Apicomplexan parasites, such as Plasmodium spp., rely on an unusual actomyosin motor, termed glideosome, for motility and host cell invasion. Actin filament capping proteins (CPs) are indispensable heterodimeric regulators of actin dynamics. CPs play a crucial role in actin dynamics by binding to the fast-growing barbed end of filamentous actin (F-actin) with high affinity in a Ca2+-independent manner, limiting protomer exchange to the pointed end. Despite retaining several characteristics of a canonical CP, the homodimeric Plasmodium berghei (Pb)CP exhibits crucial differences to the canonical heterodimers.

To gain structural insight into the unusual homodimerization of PbCPαα, we determined the structure of a C-terminally truncated PbCPαα homodimer (PbCPααΔC20), which was the only version of the parasite CPs that produced well-diffracting crystals, to 2.2-Å resolution. The two PbCPαΔC20 subunits form a structure that is less compact and intertwined than the canonical heterodimer, verifying earlier small-angle X-ray scattering (SAXS) and thermal stability analyses. Albeit being a homodimer, the structure is not completely symmetric. Thus, we will refer to chain A of the crystal structure as PbCPα1ΔC20 and chain B as PbCPα2ΔC20. Superposition of the two subunits reveals that structural deviations are mainly present at the dimer interface, possibly to accommodate complementary intersubunit interactions. In PbCPαΔC20, the presence of two identical stalk domains disrupts the formation of a compact structure. The 23-residue Plasmodium CPα-specific insert is located between the globule and cap β-sheets (Ser136–Ala159). The base of the insert is stabilized by a partial disulfide bond between Cys158 and Cys179 in the PbCPα1ΔC20 subunit but not in PbCPα2ΔC20. The H5 helix of PbCPα1ΔC20 is broken at His267 and turns back towards the same subunit in a β-hairpin-like structure (Leu268-Leu286), instead of extending into PbCPα2ΔC20, resulting in very different C termini in the subunits. Residues of the basic patch in PbCPααΔC20 are more buried in the structure, not in close proximity to each other, and the slight asymmetry of the homodimer does not compensate significantly for the loss of contributing residues of PbCPβ.

>MDSLLNEKKKFIRHVLSNAPPGKVFDLISNLKTIFGSNAIIQNFIEDIISKYNEDNYILIPFESDEYIIICKESKSGNLYLHPNLKILANVNHLKRKVIDTTPLTKLDHPDILEKYRVACNNKLKEYVDIYYKKWSDHQTGNYPTVNIGSKHGLNVKCASSVYASECENKYNLFLLICCDRYYLKNFHASSWRSSWNVNFLEADQEIILTGTIDVVLTYFEDANINFKTRKVFEKRVSVTNDIENFASSILSVIRECENDVLYDLNHLIANTSSDLIKNTRKIIPLNAHHHHHH[2x]>MGSDKIHHHHHHMYLMNTYSRFPATFVYGKGSWIYDEKGNAYLDFTSGIAVNVLGHSHPRLVEAIKDQAEKLIHCSNLFWNRPQMELAELLSKNTFGGKVFFANTGTEANEAAIKIARKYGKKKSEKKYRILSAHNSFHGRTLGSLTATGQPKYQKPFEPLVPGFEYFEFNNVEDLRRKMSEDVCAVFLEPIQGESGIVPATKEFLEEARKLCDEYDALLVFDEVQCGMGR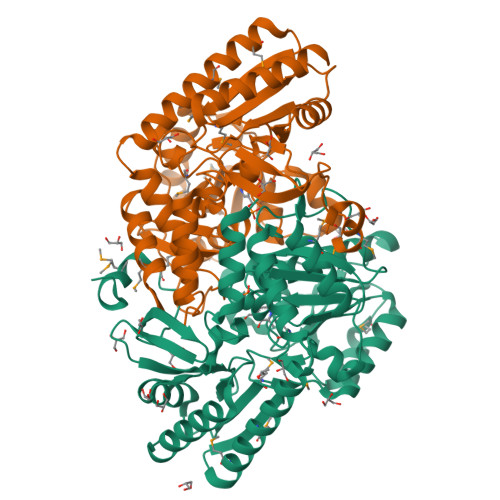TGKLFAYQKYGVVPDVLTTAKGLGGGVPIGAVIVNERANVLEPGDHGTTFGGNPLACRAGVTVIKELTKEGFLEEVEEKGNYLMKKLQEMKEEYDVVADVRGMGLMIGIQFREEVSNREVATKCFENKLLVVPAGNNTIRFLPPLTVEYGEIDLAVETLKKVLQGI[2x]>MAHHHHHHMPDTSDPRPTILLVGASRGLGHAMAAEFLKRGWDVVGTVRADRGRTPLHALAEAYPDRLRIETLDITQPEQIRALAARLSGRVFDILFVNAGTTNPDPTQTIGEVSTDDFVDLMITNALSPMRVVETLAGLVPRDGLIGIMSSGQG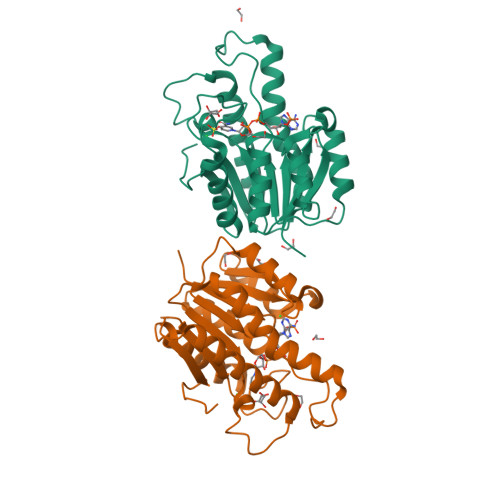SIADNESGQRELYRGSKAALNQFMRSFAARHAQTPLAMVLIAPGWVRTELGGPDARLSIDESVPGVVDVLLAKRGRAGLEYLDYRGRTVRW[2x]In low G + C Gram-positive bacteria, CodY is a global regulatory protein that controls the transcription of numerous genes. CodY from B. subtilis and most other low G + C Gram-positive bacteria is a DNA-binding protein that is activated by the branched-chain amino acids (BCAAs),2 leucine, isoleucine and valine, which may be viewed as signals of the metabolic status of the cell, and GTP, which may signal the energetic status of the cell. CodY from B. subtilis consists of 259 amino acid residues. The structures of full-length CodY from B. subtilis determined here reveal the effector binding domain and the DNA binding domain as discrete entities separated by a helical linker.

We have solved the structure of unliganded CodY in three different crystal forms containing 14 (form A), 10 (form B), and 2 (form C) molecules in the asymmetric unit from data sets extending to 4.6, 3.0, and 3.7 Å spacing, respectively. The following descriptions relate to the structure of the form B crystals, because these crystals diffracted to the highest resolution (3.0 Å). The full-length CodY protomer has an elongated structure that spans 80 Å in the longest dimension with a dumb-bell shape. The 12 residues (156–167) that link the previously reported GAF and wHTH domain structures are in an α-helical conformation. They extend helix α5 in the GAF domain and connect it to what was previously named helix α6 in the wHTH domain, thereby creating a single α-helix spanning residues 137–177. Within the CodY chain, there are no non-covalent interactions between the domains that exist as discrete entities. Examination of the molecular packing in the crystals of unliganded CodY reveals that the basic building block of all three crystals is a tetramer. The GAF domains exist as two pairs of dimers flanking four wHTH domains. To facilitate comparison, we superimposed the wHTH domains of one of the chains (chain A) of unliganded CodY and Ile-bound CodY(L3S) onto one of the corresponding domains of QsrR, FadR, and IscR in their DNA complexes and observed the juxtaposition of the recognition helix in the partner wHTH domains and the DNA. This simple modeling suggests that the unliganded CodY dimer, in which the recognition helices from each chain are related by a 25 Å translation and a 40° rotation, could bind to a DNA duplex of ∼20 bp.

>ALLQKTRIINSMLQAAAGKPVNFKEMAETLRDVIDSNIFVVSRRGKLLGYSINQQIENDRMKKMLEDRQFPEEYTKNLFNVPETSSNLDINSEYTAFPVENRDLFQAGLTTIVPIIGGGERLGTLILSRLQDQFNDDDLILAEYGATVVGMEILREKAEEIEEEARSKAVVQMAISSLSYSELEAIEHIFEELDGNEGLLVASKIADRVGITRSVIVNALRKLESAGVIESRSLGMKGTYIKVLNNKFLIELENLKSHHHHHH[10x]> MENVVSAPMPGKVLRVLVRVGDRVRVGQGLLVLEAMKMENEIPSPRDGVVKRILVKEGEYVDTGQPLIELG

We previously determined the crystal structure of the C-terminal 73-residue fragment of PhBCCP (PhBCCPΔN76) that represents the biotinyl(/lipoyl attachment) domain of the hypothetical methylmalonyl-CoA decarboxylase γ chain. This domain adopts a flattened β-barrel comprising two homologous ‘hammerhead’ structures that confer an intramolecular pseudo-twofold symmetry reflecting the gene duplication. In this work, we used the C-terminal 70-residue fragment of PhBCCP (PhBCCPΔN79) as the template to prevent the N-terminal heterogeneity that was observed in PhBCCPΔN76. Moderate deviations of up to 2.53 Å were observed at residues 114–116, which constitute a flexible β-turn harbouring the Lys115 residue to be biotinylated.

In the PhBCCP system (PhBCCPΔN79) residue 138 was selected as the target residue for the mutation experiment because it is a solvent-exposed and nonconserved residue on a surface β-sheet. The isoleucine mutant (A138I) and the tyrosine mutant (A138Y) conferring residue 138 with the highest crystal-packing propensities for β-sheet provided better crystallization scores when compared with other constructs, including the wild type. The A138I mutant and the A138Y mutant produced another orthorhombic crystal form belonging to space group C2221 and a trigonal crystal form belonging to space group P3121, respectively. The crystal structures of the A138I and A138Y mutants were determined at resolutions of 1.9 and 1.5 Å, respectively. In these mutant crystals the crystal-packing interface involving residue 138 differs completely from those of the other two crystal forms. Neither the C orthorhombic nor the trigonal crystals could be obtained with the wild-type protein. Therefore, it is conceivable that the substitution of Ala by Ile/Tyr with a better crystal-packing propensity created novel packing interfaces. On the other hand, the crystal packings of the A138I and A138Y mutants are rich in attractive electrostatic interactions and nonpolar interactions, respectively. The numbers of nonpolar interactions normalized by the total buried ASA for the three crystal forms were calculated as 0.108 Å−2 for the wild type, 0.099 Å−2 for the A138I mutant and 0.135 Å−2 for the A138Y mutant. The order of the normalized number of nonpolar interactions corresponds to that of the resolution.> MPRPRVLLLGDPARHLDDLWSDFQQKFEVIPANLTTHDGFKQALREKRYGDFEAII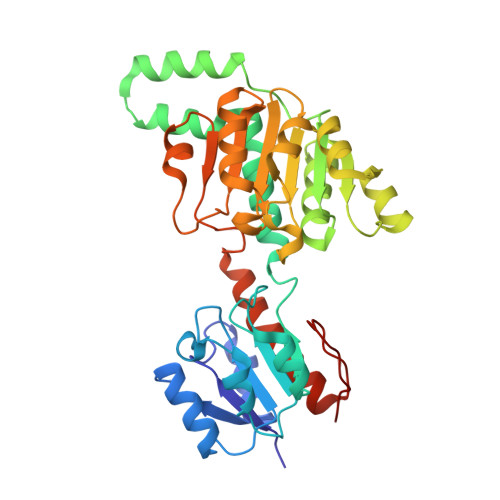KLAVENGTESYPWNADLISHLPSSLKVFAAAGAGFDWLDLDALNERGVAFANSRGAGDTATSDLALYLILSVFRLASYSERAARTGDPETFNRVHLEIGKSAHNPRGHVLGAVGLGAIQKEIARKAVHGLGMKLVYYDVAPADAETEKALGAERVDSLEELARRSDCVSVSVPYMKLTHHLIDEAFFAAMKPGSRIVNTARGPVISQDALIAALKSGKLLSAGLDVHEFEPQVSKELIEMKHVTLTTHIGGVAIETFHEFERLTMTNIDRFLLQGKPLLTPAGKVFAPSSAA> AFVVTDNCIKCKYTKCVEVCPVDCFYEGPNFLVIHPDE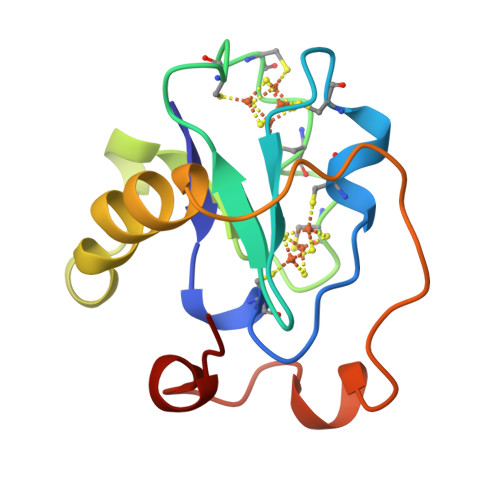CIDCALCEPECPAQAIFSEDEVPEDMQEFIQLNAELAEVWPNITEDKDPLPDAEDWDGVKGKLQHLER>APSRKFFVGGNWKMNGRKQSLGELIGTLNAAKVPADTEVVCAPPTAYIDFARQKLDPKIAVAAQNCYKVTNGAFTGEISPGMIKDCGATWVVLGHSERRHVFGESDELIGQKVAHALAEGLGVIACIGEKLDEREAGITEKVVFEQTKVIADNMKDWSKVVLAYEPVWAIGTGKTATPQQAQEVHEKLRGWLKSNVSDAVAQSTRIIYGGSVTGATCKELASQPDVDGFLVGGAS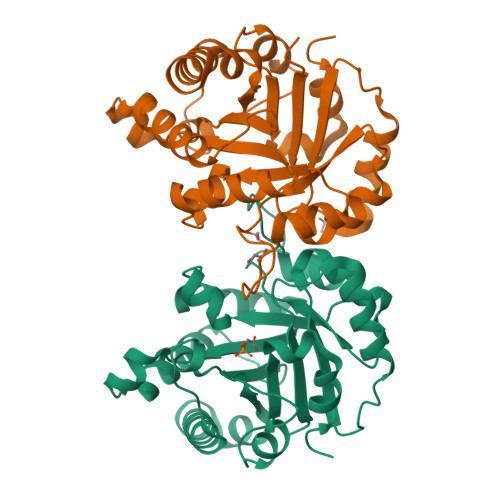LKPEFVDIINAKQ[2x]> MSSSLLSVLKEKSRSLKIRNKPVKMTSQERMI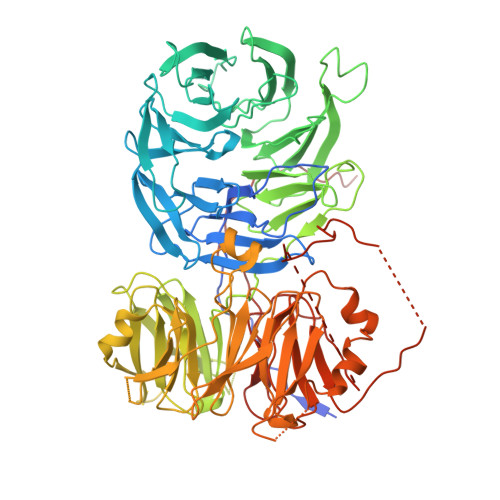VHRCRFVDFTPATITSLAFSHKSNINKLTPSDLRLAIGRSNGNIEIWNPRNNWFQEMVIEGGKDRSIEGLCWSNVNGESLRLFSIGGSTVVTEWDLATGLPLRNYDCNSGVIWSISINDSQDKLSVGCDNGTVVLIDISGGPGVLEHDTILMRQEARVLTLAWKKDDFVIGGCSDGRIRIWSAQKNDENMGRLLHTMKVDKAKKESTLVWSVIYLPRTDQIASGDSTGSIKFWDFQFATLNQSFKAHDADVLCLTTDTDNNYVFSAGVDRKIFQFSQNTNKSQKNNRWVNSSNRLLHGNDIRAICAYQSKGADFLVSGGVEKTLVINSLTSFSNGNYRKMPTVEPYSKNVLVNKEQRLVVSWSESTVKIWTMGTDSSTEQNYKLVCKLTLKDDQNISTCSLSPDGQVLVVGRPSTTKVFHLQPVGNKLKVTKLDNDLLLRTSTKLVKFIDNSKIVICSCEDDVFIVDLESEEDEKPQEVELLEVTSTKSSIKVPYINRINHLEVDQNIAVISRGCGVVDILDLKARISKPLARLNNFITAVHINTSRKSVVVITADNKIYEFNMNLNSEAENEDSESVLTQWSKNNTDNLPKEWKTLKENCVGIFSDIENSSRLWFWGATWISRIDFDVDFPINKXXXXXXXXXXXXXXHFFFTDKYKPLLFVDLISSNELAIIERNPLTFHSKQKAFIQPKLVF> MGAQVSTQKSGSHETGNVATGGSTINFTNINYYKDSYAASATRQDFTQDPKKFTQPVLDSIRELSAPLNSPSVEACGYSDRVAQLTVGNSSITTQEAANIVLAYGEWPEYCPDTDATAVDKPTRPDVSVNRFYTLDSKMWQENSTGWYWKFPDVLNKTGVFGQNAQFHYLYRSGFCLHVQCNASKFHQGALLVAVIPEFVIAGRGSNTKPNEAPHPGFTTTFPGTTGATFHDPYVLDSGVPLSQALIYPHQWVNLRTNNCATVIVPYINAVPFDSAINHS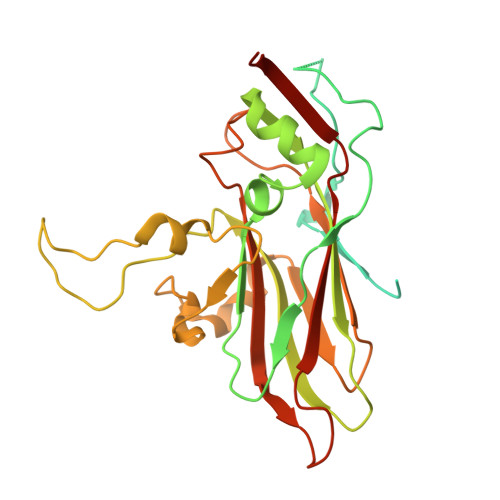NFGLVVVPVSPLKYSSGATTAIPITITIAPLNSEFGGLRQAVSQ> PDQFRAIIESPEGAGHVGYQYRRNTGSTMRMVSDVLDERVSLWDFHCDPSGNVIQPGPNVDSRQYLQAAIDYVSSNGGGTITIPAGYTWYLGSYGVGGIAGHSGIIQLRSNVNLNIEGRIHLSPFFDLKPFQVFVGFDNGDPASSGNLENCHIYGHGVVDFGGYEFGASSQLRNGVAFGRSYNCSVTGITFQNGDVTWAITLGWNGYGSNCYVRKCRFINLVNSSVNADHSTVYVNCPYSGVESCYFSMSSSFARNIACSVQLHQHDTFYRGSTVNGYCRGAYVVMHAAEAAGAGSYAYNMQVENNIAVIYGQFVILGSDVTATVSGHLNDVIVSGNIVSIGERAAFSAPFGAFIDIGPDGASNVQDIQRVLVTGNSFYAPANITDSAAITLRANLNGCTFIANNFDCRYMVYNAPGTTSPVVQNLVWDKSNVIGGTHANQRAGQNLFDMQFASVVNSTIEVQLSCEDLSMFSCILFPASCQLSYSKITVDSAWTKSMSNTAVFEGN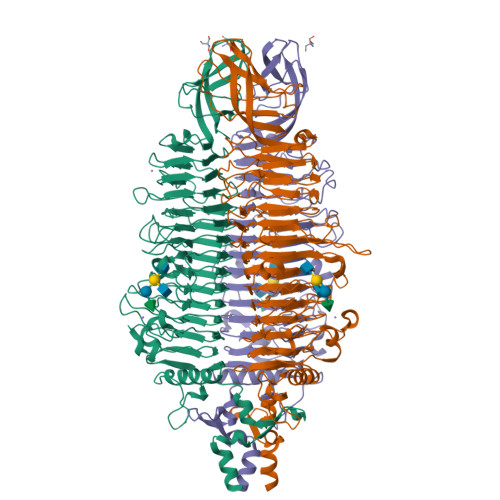QQAGANVYVSYPATVNLTSYNTQGAVPFFSTDTNYAWVTSAYSLSINENLDFSPPATYTNKANGQLVGVGYNEIGGVRSVSVRLMLQRQV> NSVFSGLDMLILLPYERRGTRLVVEDYRPDHIYCIGADFGKNQDYSVFSVLDLDTGAIACLERMNGATWSDQVARLKALSEDYGHAYVVADTWGVGDAIAEELDAQGINYTPLPVKSSSVKEQLISNLALLMEKGQVAVPNDKTILDELRNFRYYRTASGNQVMRAYGRGHDDIVMSLALAYSQYEG

The large terminase protein is a key component of the DNA packaging machinery in tailed bacteriophages and evolutionarily related herpes viruses. Typically, in addition to an ATPase domain which powers DNA translocation, the large terminase contains a nuclease domain which cuts concatemeric DNA, generated by rolling circle replication. Crystal structures of the large terminase nuclease from the thermophilic bacteriophage G20c show that it is most similar to the RuvC family of the RNase H-like endonucleases. The overall structure adopts the RNase-H fold.

Initial crystals were obtained from a proteolytically cleaved C-terminal fragment of the full-length protein (Crystal form 1). A bound Zn2+ ion from the crystallization solution enabled the structure to be determined by SAD. Only one metal ion, bound to the site A, was identified for conditions containing Mg2+, Mn2+ and Co2+. This metal ion is coordinated by the side chains of D294 and D429 and four water molecules in the canonical octahedral geometry. A similar coordination is observed for Zn2+, although there is also a second Zn2+ ion bound at an additional satellite site, at a distance of 4.6 Å from the site A Zn2+ ion. Superposition of the G20c nuclease structure containing two Zn2+ ions (Crystal form 1) with SPP1 G2P and HCMV UL89 nucleases containing two bound Mn2+ ions shows that while one Zn2+ ion is bound at site A, the second Zn2+ ion is bound on the opposite side of site B. This Zn2+ ion is in a tetrahedral coordination with D429, H427, D300 and a solvent molecule. In our structure, complexed with two Zn2+ ions, the Zn2+ ion bound at catalytic site A adopts an octahedral geometry, resembling the canonical coordination of Mg2+ that would support catalysis. However, the second Zn2+ bound at an adjacent binding site, not previously reported for the RNase H-like endonucleases, is coordinated by catalytically important residues D429 and H427. Binding of this second Zn2+ ion perturbs charge distribution in the active site and may affect DNA and metal B binding as well as water nucleophile formation and coordination.> QLYSALANKCCHVGCT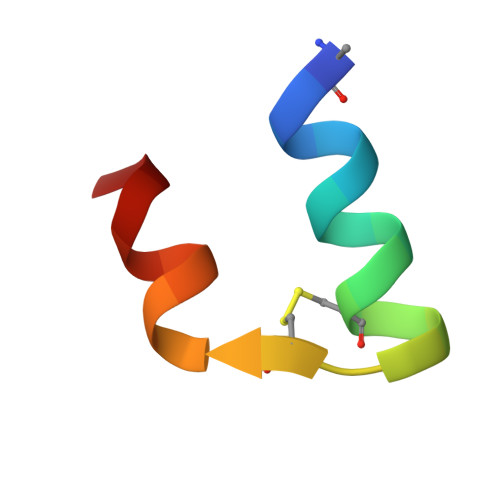KRSLARFC Here we characterize a set of compact CRISPR-Cas12m (subtype V-M) effector proteins and show that they provide protection against bacteriophages and plasmids through the targeted DNA binding rather than DNA cleavage. Biochemical assays suggest that Cas12m effectors can act as roadblocks inhibiting DNA transcription and/or replication, thereby triggering interference against invaders. Sequence analysis of enriched RNAs derived from regions adjacent to the CRISPR array did not reveal complementarity to the repeat sequences, ruling out the presence of the trans-activating RNAs (tracrRNAs) and indicating that Cas12m proteins are guided to the DNA target by a single short (50–60 nt) crRNA. Here we show that DNA-binding activity without cleavage is a common feature of the Cas12m effectors, thereby expanding our understanding of the functionally diverse type V Cas12 protein family.

To better understand the molecular mechanism of DNA silencing by Cas12m effectors, we have determined the structure of GoCas12m bound to crRNA and target DNA using cryogenic-electron microscopy (cryo-EM). The 2.93 Å structure of GoCas12m-crRNA-DNA ternary complex revealed that GoCas12m protein adopts a bi-lobed structure, characteristic to other Cas12/TnpB proteins, consisting of the N-terminal recognition (Rec) and C-terminal nuclease (Nuc) lobes. The Rec lobe contains wedge (WED) and REC domains, while the Nuc lobe includes a RuvC-like domain with an unusual H322-D497-D590 triad at the active site and a Zinc finger (ZnF) domain. In comparison to TnpB, which comprises the minimal functional core of the Cas12 nuclease family, Cas12m has acquired a long ɑ-helical insertion (termed ‘Roof’) in the REC domain (residues 50–124), a larger ɑ-helical subdomain between the ꞵ11- and ꞵ12-strands of the RuvC domain, and several insertions in the WED domain. The ∼30 nt CRISPR repeat-derived GoCas12m crRNA fragment folds into a compact structure consisting of a triplex region and a pseudoknot (PK), which is anchored to GoCas12m WED and RuvC domains by hydrogen bond (H-bond) and van der Waals (vdW) contacts. The 5′-TTN-3′ PAM-containing region of the target dsDNA is accommodated between the REC and WED domains. All four bases of the 5′-TT-3′ dinucleotide are read out through base-specific H-bond and vdW contacts. Separation of the target (TS) and non-target (NTS) DNA strands immediately downstream of the PAM is facilitated by the REC domain residues Y134 and N156 that insert between the two strands and stabilize the last unseparated DNA base pair. The guide RNA-TS DNA heteroduplex is enclosed between the Nuc and Rec lobes and is stabilized by multiple interactions between the phosphodiester backbone and residues from the WED and RuvC domains, similar to the smaller TnpB enzyme.

> SNAGGGGMTRVTVQTAGVHYKWQMPDQLTQQLRLAHDLREDLVTLEYEYEDAVKAVWSSYPAVAALEAQVAELDERASELASTVKEEKSRQRTKRPSHPAVAQLAETRAQLKAAKASRREAIASVRDEATERLRTISDERYAAQKQLYRDYCTDGLLYWATFNAVLDHHKTAVKRIAAHRKQGRAAQLRHHRWDGTGTISVQLQRQATDPARTPAIIADADTGKWRSSLIVPWVNPDVWDTMDRASRRKAGRVVIRMRCGSSRNPDGTKTSEWIDVPVQQHRMLPADADITAAQLTVRREGADLRATIGITAKIPDQGEVDEGPTIAVHLGWRSSDHGTVVATWRSTEPLDIPETLRGVITTQSAERTVGSIVVPHRIEQRVHHHATVASHRDLAVDSIRDTLVAWLTEHGPQPHPYDGDPITAASVQRWKAPRRFAWLALQWRDTPPPEGADIAETLEAWRRADKKLWLESEHGRGRALRHRTDLHRQVAAYFAGVAGRIVVDDSDIAQIAGTAKHSELLTDVDRQIARRRAIAAPGMLRAAIVAAATRDEVPTTTVSHTGLSRVHAACGHENPADDRYLMQPVLCDGCGRTYDTDLSATILMLQRASAATSN> GGFAQIYTVKAGDSIYSIAKQFRIDAGKIIRANELPNPNQLVIGQSMVIPINGTYYTVKAGDTIWKVGRKLGVSYQAIANANNVSVTAPLTPGRRILIPPSPNKRNGEFLGYVETSNRKITPQTEKMINQNAKYLTYLGPANFEVQKDGSLKAPPLNNLGSIAKENDVIFLMVLANIENGAFSDEV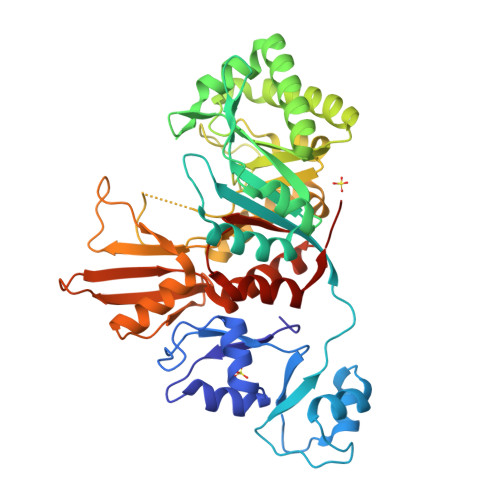GRAILNNKDVQDTLLNNIVKTAKEQNFRDIHFDFEFLRPADKEAYIAFLQKAKKRLQDEQLLMSVALAPKTSRDQKGKWYEAHDYKAIGEIANFVVPMTYEWGYSGGPPMAVSPIGPVRDVLEYAVSEIPSSKIIMGQNLYGYDWTLPYKPGGEYAKAISPQRAIELAARYKVAIQYDNKAQAPFFRYKDEQQRTHEVWFEDARSIQAKFDLIKELKLRGMAYWKLGLDFPQNWLLIEDNFKITKRVTQP The DENV lipid envelope contains 180 copies of the envelope glycoprotein (E), which covers the surface of the virus particle. On the mature infectious virus particle, E is arranged in a herringbone pattern as antiparallel homodimers that pack laterally into a lipid raft containing three dimers. The E protein monomer contains three predominantly β sheet domains (DI, DII, and DIII) connected to a transmembrane domain by an amphipathic helix. As DENV enters the cell, the E protein undergoes a pH-induced conformational change from a dimeric to a trimeric form that triggers fusion of viral and endosomal membranes required for releasing the viral genome into the cytoplasm of the cell.

Variant SC.10, which builds on SC.14 with a single additional mutation G106D (IntFc8), further raised Tm1 to 53.9°C and lowered the Kd to less than 100 pM at 37°C. The exceptional stability of the SC.10 dimer is likely due to simultaneously stabilizing the central dimer interface (IntFc2), the hinge (UndPk6), and the FL dimer interface (IntFc8), all critical regions that regulate dimer stability. To compare SC.10 and WT sE structures and to validate the accuracy of the Rosetta design models, we determined the crystal structure of SC.10 at 3.42 Å using molecular replacement (MR). Despite growing the crystal at pH 4.4, SC.10 retained the prefusion DENV2 sE dimer conformation. The SC.10 crystal structure follows this pattern and has a DI/DII hinge angle that supports a conformation that is flatter than what is observed on the virion. However, these changes do not appear to have a large influence on the binding of potently neutralizing EDE1 human monoclonal antibodies because the WT DENV2 sE protein crystallized with EDE1 antibodies adopts a conformation that is similar to the structure we observed for SC.10 (16, 36). In addition to the structural rigidity that prolines can provide, the new hydrogen bond may be helping to stabilize the sE dimer. As predicted by the Rosetta model, the two mutations in IntFc2, T262R and A259W, lead to canonical pi-cation interactions across the central dimer interface between R262 on one chain and W259 on the other chain. The two UndPk6 mutations, F279W and T280P, are in the kl loop of the DI/DII hinge. T280P is at the base of the kl loop, and in the SC.10 structure, the backbone at residue 280 is shifted to create a new backbone side chain hydrogen bond between the P280 backbone carbonyl and the T189 side chain hydroxyl in an adjacent loop. Instead, in the SC.10 structure, D106 forms an intradomain hydrogen bond with Q77, and alternative rotamers are observed for K310 and W101.

> MRCIGMSNRDFVEGVSGGSWVDIVLEHGSCVTTMAKNKPTLDFELIKTEAKQPATLRKYCIEAKLTNTTTESRCPTQGEPSLNEEQDKRFVCKHSMVDRGWGNGCDLFGKGGIVTCAMFRCKKNMEGKVVQPENLEYTIVITPHSGEEHAVGNDTGKHGKEIKITPQSSITEAELTGYGTVTMECSPRTGLDFNEMVLLQMENKAWLVHRQWFLDLPLPWLPGADTQGSNWIQKETLVTFKNPHAKKQDVVVLGSQEGWMHRALTGATEIQMSSGNLLWPGHLKCRLRMDKLQLKGMSYSMCTGKFKVVKEIAETQHGTIVIRVQYEGDGSPCKIPFEIMDLEKRHVLGRLITVNPIVTEKDSPVNIEAEPPFGDSYIIIGVEPGQLKLNWFKKGSSGGSHHHHHHHH The adherence of UPEC to the urothelial surface is mediated through the mannose-specific lectin FimH, the natural ligand of which is the mannosylated glycoprotein uroplakin Ia present on urothelial cells. Mannose-based FimH antagonists compete with this interaction and prevent bacterial adhesion and hence infection. Here, the first crystal structures of C-glycosidically linked α-d-mannopyranosides in complex with the FimH adhesin of uropathogenic E. coli J96 are reported. Two ligands are decorated with a para-biphenyl group on a C-linkage to an ethene spacer (CcbP) or to an ethene with a branched methyl spacer (CtbP) and one with a naphthyl group on a C-linkage to an ethyl spacer (CN).

After several cycles of isotropic temperature-factor refinement, we solved the three-dimensional structure of the FimH–CtbP complex with one molecule in the asymmetric unit. CtbP is bound to the N-terminal region of FimH with the mannose ring tightly bound in a hydrophilic pocket able to stabilize the sugar moiety. Indeed, multiple hydrogen bonds are formed to amino acids such as Asn46, Asn135 and Asp140 and also water molecules. Owing to the trans stereochemistry of the 1E ethene group, the biphenyl part of the ligand accommodates the closed tyrosine gate formed by Tyr48 (χ1 = −164.0°, χ2 = −169.2°) and Tyr137. Moreover, the hydrophobic biphenyl moiety also interacts with the lipophilic amino acids Pro26 and Val27 of a neighbouring FimH molecule because of the crystal packing. Despite the hydrophobic pattern of CtbP, this ligand is solvated with well structured water molecules (average B factor of 18.5 Å2) on its solvent-exposed side. CtbP (trans) and CcbP (cis) can accommodate both open and closed conformations of the tyrosine gate formed by Tyr48 and Tyr137. We found that the linker-associated water molecule is shifted away from the C-glycosidic linkages compared with the O- and N-glycosidic linkages and that another water molecule could come in to assist in hydrogen bonding downstream of the C-glycosidic bond.

> FACKTANGTAIPIGGGSANVYVNLAPVVNVGQNLVVDLSTQIFCHNDYPETITDYVTLQRGSAYGGVLSNFSGTVKYSGSSYPFPTTSETPRVVYNSRTDKPWPVALYLTPVSSAGGVAIKAGSLIAVLILRQTNNYNSDDFQFVWNIYANNDVVVPT The RGD (Arg-Gly-Asp)-binding integrins αvβ6 and αvβ8 are clinically validated cancer and fibrosis targets of considerable therapeutic importance. The highly homologous integrins αvβ6 and αvβ8 bind to latent transforming growth factor-β1 and β3 (L-TGF-β1 and L-TGF-β3) leading to release of active TGF-β1 and -β31–3. Here, we describe a method for computationally designing hyperstable RGD-containing miniproteins that are highly selective for a single RGD integrin heterodimer and conformational state, and use this strategy to design inhibitors of αvβ6 and αvβ8 with high selectivity. We found small α/β ferredoxin folds were able to scaffold the RGDLXX(L/I) binding loop without clashing with the integrin while making additional contacts with both α and β subunit (α- and β-loop respectively).

For the ease of aerosol formulation, we sought to increase the stability of the engineered inhibitors. Four variants with additional disulfide bonds stapling the N and C terminus had considerably increased thermostability, and bound to αvβ6 with subnanomolar affinity; mutation of the RGD to KGE abrogated binding to αvβ6 confirming that the RGD loop is necessary for binding. For αvβ6 integrin, B6_BP_dslf had the lowest IC50 (1.84 nM), followed by B6B8_BP_dslf (3.79 nM), PLN-74809 (4.36 nM); B8_BP_dslf had no detectable binding consistent with its very high selectivity. Taken together, these data confirm that B6_BP_dslf and B8_BP_dslf have exquisite selectivity and affinity for their respective integrin targets, with considerably greater RGD integrin selectivity than the small molecules PLN-74809 and GSK3008348. We also characterized the pharmacokinetics of B6_BP_dslf in the lungs and serum of healthy male C57BL/6 mice following a single dose via different routes of administration. B6_BP_dslf was rapidly cleared from the blood following IV and IP administration with a half-life of ~10 min, and following inhaled administration, B6_BP_dslf had a half-life in the lungs of ~1 h. The properties of B6_BP_dslf are unchanged following aerosolization: the protein is monomeric, thermostable, has the same CD spectrum, and binds to αvβ6 with similar affinity. In addition to the highly potent anti-fibrotic effects demonstrated here in the bleomycin-induced lung fibrosis model, the reduced systemic exposure due to the short serum half-life (~10 min), high selectivity and affinity for αvβ6, stabilization of the open αvβ6 conformation, ease of production using E. coli, hyper-thermostability, and aerosol formulatability give B6_BP_dslf an improved target product profile as a therapeutic candidate for IPF.

>[3x]STKCVVRFVFRGDLATLMLRAVKDHLKKEGPHWNITSTNNGAELVVRGIHESDAKRIAKWVEKRFPGVHTETQCD> MGSLVCVGTGLQLAGQISVLSRSYIEHADIVFSLLPDGFSQRWLTKLNPNVINLQQFYAQNGEVKNRRDTYEQMVNAILDAVRAGKKTVCALFGHPGVFACVSHMAITRAKAEGFSAKMEPGISAEACLWADLGIDPGNSGHQSFEASQFMFFNHVPDPTTHLLLWQIAIAGEHTLTQFHTSSDRLQILVEQLNQWYPLDHEVVIYEAANLPIQAPRIERLPLANLPQAHLMPISTLLIPPAKKLE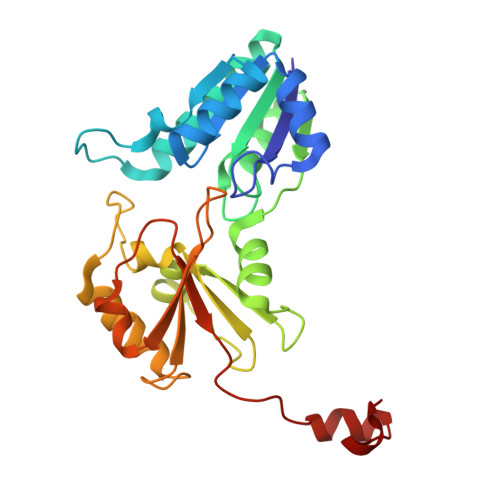YNYAILAKLGIGPEDLG>MAKIYTDKDVSLDVIKEKRVAVLGYGSQGRAWALNLRDSGIKVSVGLEREGNSWKQAENDGFKPLRTEEAVRNSDIIIFLLPDMIQRTVYLERVKPYLKEGMDLVFAHGFNIHYRLIEPPSNVDVYMIAPKAPGPIVREYFAKGGGVPALVATYQDHSGKALQKALAVAKAIGATRAGVIETTFKEETETDLFGEQVDLVGGVMQLMRYAFQTLVEAGYQPEVAYFETINEMKLIVDLVYEKGFSGMLTAVSDTAKYGGMTVGKMVIDESVKERMKKALDNIRSGKFAEKWVEEYGKGANTIKEGMKEVDNSTEEKVGRSLRDIILRGKPKSLEHHHHHH[2x]

The BCAAs are synthesized from pyruvate by a common pathway that involves acetolactate synthase (ALS), ketol-acid reductoisomerase (KARI), and dihydroxy-acid dehydratase (DHAD). As a bifunctional key enzyme, KARI catalyzes an essential two-step reaction for BCAA biosynthesis. Proteins of both classes fold into an N-terminal Rossmann domain and a C-terminal “knot” domain.

In this study, we present the crystal structure of a class-I KARI from the thermoacidophilic archaeon Sulfolobus acidocaldarius at 1.75-Å resolution. Gel filtration showed that in the presence of 2 mM Mg2+ Sac-KARI is a dimer with a molecular weight of ~70 kDa (the theoretical molecular weight of the dimer is ~74 kDa). Each monomer of Sac-KARI folds into an N-terminal Rossmann domain and a C-terminal “knot” domain. In addition, probably because of the presence of 2 mM magnesium in the lysis and purification buffers, a Mg2+ was seen in each active site, surrounded by the side chains of E227 and E231 of one monomer and D191 of another. Mg2+ (I) is coordinated by D191 and E195 and Mg2+ (II) by D191, E227 and E231. In Sac-KARI, only Mg2+ (II) is observed. Our Sac-KARI crystal structure contains a sulphate at the cofactor binding site, implying that R49 and S53 are involved in binding the 2′-phosphate of NADPH as in Ia-KARI and Se-KARI. The Sac-KARI crystal structure shows an “open” state with the active site exposed to solvent, similar to the structures of apo-Ia-KARI and Mt-KARI-Mg2+ complex. We believe that Sac-KARI shares an induced-fit mechanism in which the active site closes upon cofactor binding that is similar to that observed in the prokaryotic class I KARIs and plant class II KARIs but distinct from that of Ec-KARI. In conclusion, Sac-KARI is one of the rare enzymes that displays high activity at elevated temperatures, a board range of pH tolerance and is able to utilize both NADH and NADPH as co-factors.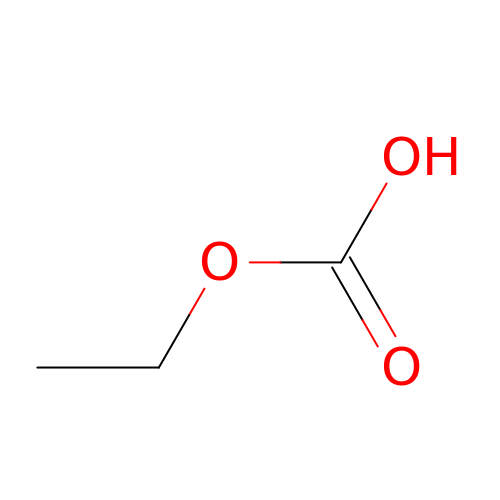ethyl hydrogen carbonate | C3 H6 O3 | CQDGTJPVBWZJAZ-UHFFFAOYSA-N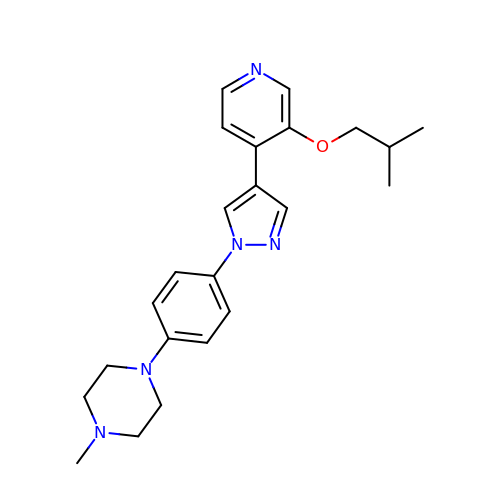1-methyl-4-(4-{4-[3-(2-methylpropoxy)pyridin-4-yl]-1H-pyrazol-1-yl}phenyl)piperazine | C23 H29 N5 O | SYZOJQFDCIIANZ-UHFFFAOYSA-N> PA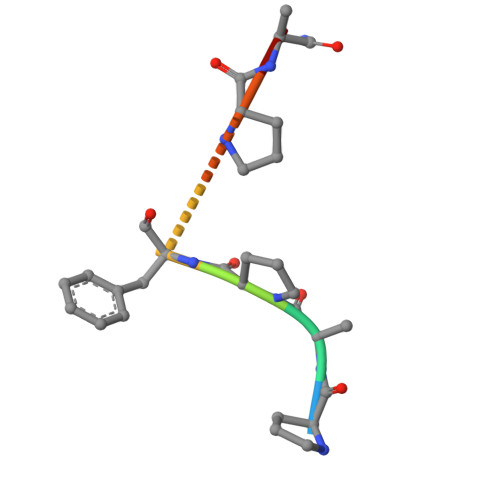PFPAX> MAEHDFETISSETLHTGAIFALRRDQVRMPGGGIVTREVVEHFGAVAIVAMDDNGNIPMVYQYRHTYGRRLWELPAGLLDVAGEPPHLTAARELREEVGLQASTWQVLVDLDTAPGFSDESVRVYLATGLREVGRPEAHHEEADMTMGWYPIAEAARRVLRGEIVNSIA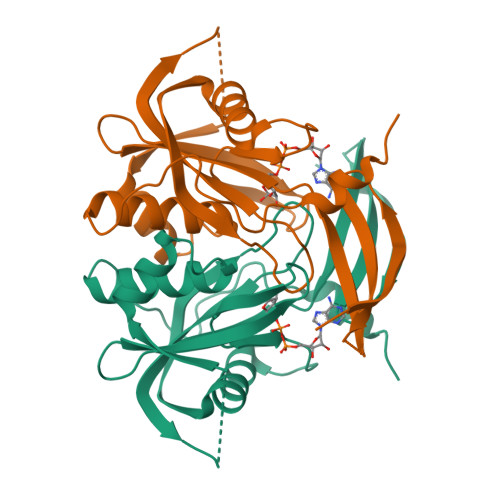IAGVLAVHAVTTGFAQPRPLDTEWIDRPTAFAARRAER> GPLGSMSNYSVSLVGPAPWGFRLQGGKDFNMPLT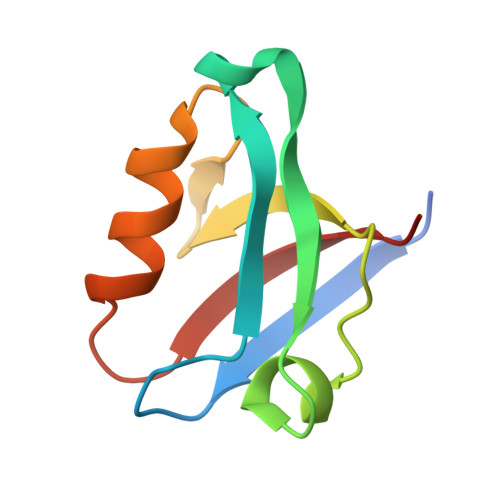ISSLKDGGKAAQANVRIGDVVLSIDGINAQGMTHLEAQNKIKGCTGSLNMTLQRAS> SKEGSVAPKERINIKYIPATGDAQAEVELPLKTLVVGDFKGHAEQTPLEERATVTVDKNNFE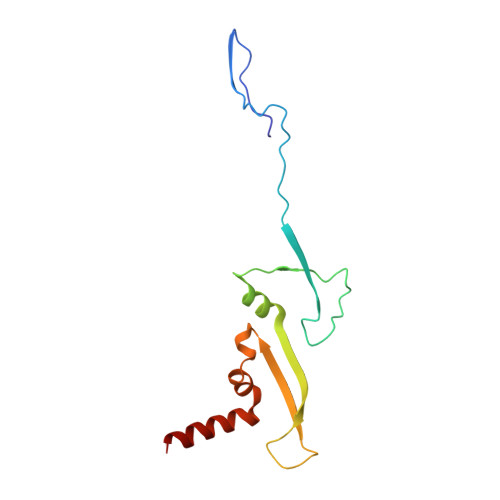AVMRESELKITATVKNKLTDDENAELPVELNFKSLADFAPDAVASQVPELKKLIELREALVAL>GHMANSVLFPCKYASSGCEITLPHTEKADHEELCEFRPYSCPCPGASCKWQGSLDAVMPHLMHQHKSITTLQGEDIVFLATDINLPGAVDWVMMQSCFGFHFMLVLEKQEKYDGHQQFFAIVQLIGTRKQAENFAYRLELNGHRRRLTWEATPRSIHEGIATAIMNSDCL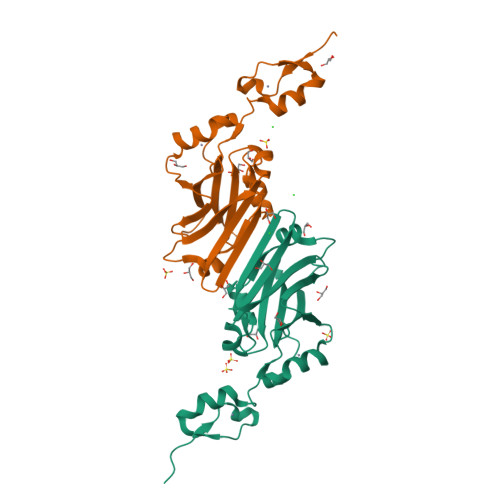VFDTSIAQLFAENGNLGINVTISMC[2x]3-HYDROXY-3-CARBOXY-ADIPIC ACID | C7 H10 O7 | 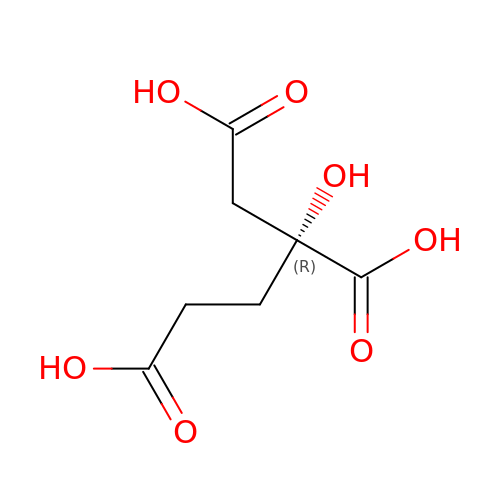XKJVEVRQMLKSMO-SSDOTTSWSA-N> ASMTGGQQMGAPITAYAQQTRGLLGCIITSLTGRDKNQVEGEVQIVSTATQTFLATCINGVCWTVYHGAGTRTIASPKGPVIQMYTNVDQDLVGWPAPQGSRSLTPCTCGSSDLYLVTRHADVIPVRRRGDSRGSLLSPRPISYLKGSSGGPL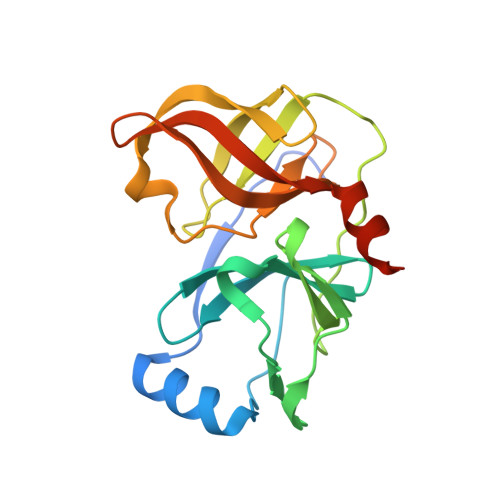LCPAGHAVGLFRAAVCTRGVAKAVDFIPVENLETTMRGSHHHHHH> GARSSSYSGEYGSGGGKRFSHSGNQLDGPITALRVRVNTYYIVGLQVRYGKVWSDYVGGRNGDLEEIFLHPGESVIQVSGKYKWYLKKLVFVTDKGRYLSFGKDSGTSFNAVPLHPNTVLRFISGRSGSLIDAIGLHW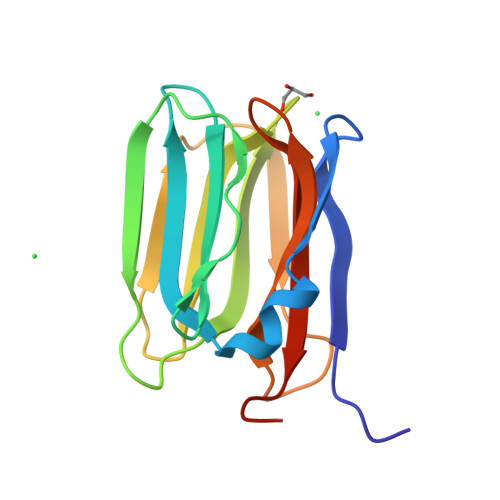DVYPSSCSRC> G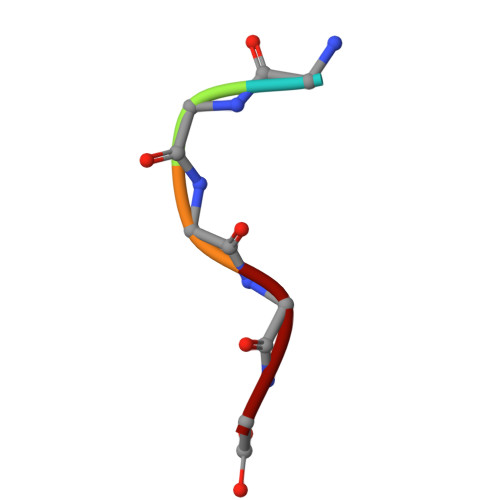GGGG> HMSLSVANSTYETTALNSQKSSTDQPNSGSKSGQTLDLVNLGVAANFAILSKT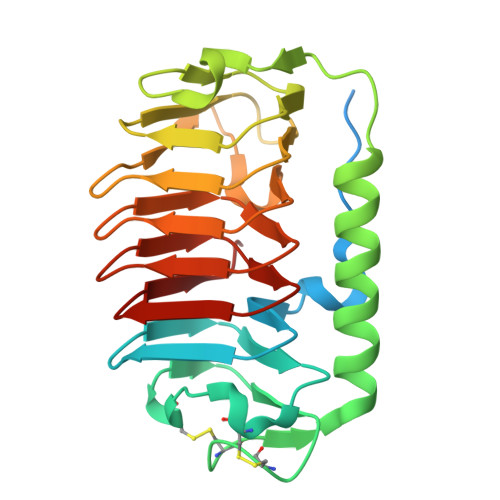GITDVYKSAITGDVGASPITGCAILLKCDEVTGTIFSVDACGPACKITDASRLTTAVGDMQIAYDNAAGRLNPDFLNLGAGTIGGKTLTPGLYKWTSTLNIPTDITISGSSTDVWIFQVAGNLNMSSAVRITLAGGAQAKNIFWQTAGAVTLGSTSHFEGNILSQTGINMKTAASINGRMMAQTAVTLQMNTVTIPQ> GPQDPTIFEERHLKYISQLGKGNFGSVELCRYDPLGDNTGALVAVKQLQHSGPDQQRDFQREIQILKALHSDFIVKYRGVSYGPGRQSLRLVMEYLPSGCLRDFLQRHRARLDASRLLLYSSQICKGMEYLGSRRCVH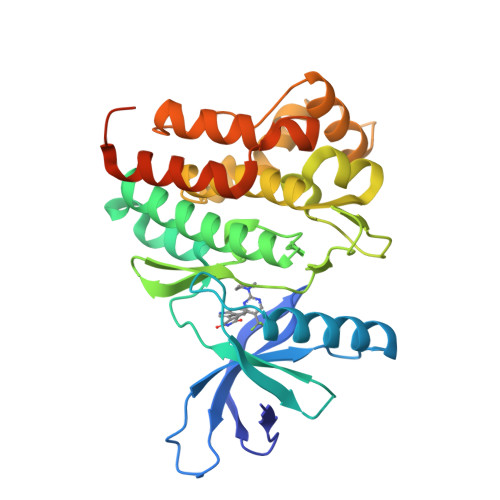RDLAARNILVESEAHVKIADFGLAKLLPLDKDYYVVREPGQSPIFWYAPESLSDNIFSRQSDVWSFGVVLYELFTYCDKSCSPSAEFLRMMGCERDVPALCRLLELLEEGQRLPAPPACPAEVHELMKLCWAPSPQDRPSFSALGPQLDMLWSGSRGCETHAFTAHPEGKHHSLSFS>[2x]SIDLSVDTSEYNRPLIHFTPEKGWMNDPNGLFYDKTAKLWHLYFQYNPNATAWG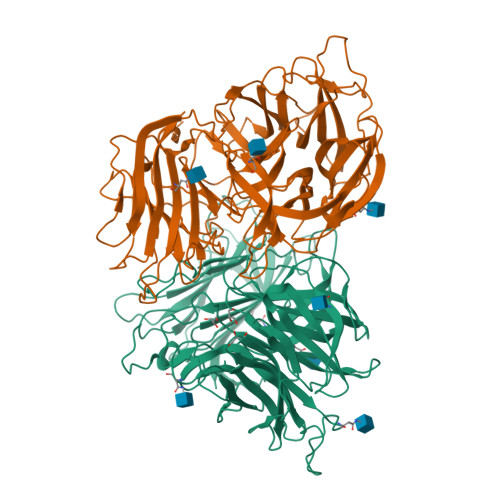QPLYWGHATSNDLVHWDEHEIAIGPEHDNEGIFSGSIVVDHNNTSGFFNSSIDPNQRIVAIYTNNIPDNQTQDIAFSLDGGYTFTKYENNPVIDVSSNQFRDPKVFWHEDSNQWIMVVSKSQEYKIQIFGSANLKNWVLNSNFSSGYYGNQYECPGLIEVPIENSDKSKWVMFLAINPGSPLGGSINQYFVGDFDGFQFVPDDSQTRFVDIGKDFYAFQTFSEVEHGVLGLAWASNWQYADQVPTNPWRSSTSLARNYTLRYVHTNAETKQLTLIQNPVLPDSINVVDKLKKKNVKLTNKKPIKTNFKGSTGLFDFNITFKVLNLNVSPGKTHFDILINSQELNSSVDSIKIGFDSSQSSFYIDRHIPNVEFPRKQFFTDKLAAYLEPLDYDQDLRVFSLYGIVDKNIIELYFNDGTVAMTNTFFMGEGKYPHDIQIVTDTEEPLFELESVIIRELNK> MFKNAKEFVQYANKLKTLREKKLNGVSIYVCVGTGCTAKGALKVYSAFEEELKKRNLLGQVTLEKIDDDKVTLNRTGCCGRCSSGPLVKIMPYRFFYSNVAPEDVPEIVDRTVLKGEPIERLFLTDPLTGEKVPRIEDTTLFKNQDFYIMEAIGESECDSIEDYIARSGYESLVKALTSMTPEEIIETVKASGLRGRGGGGFPTGLKWEFTRKAQGDIKFVVCNGDEGDPGAFMNRTLLERDPHLVLEGMIIAGYAVGAQKGYAYIRAEYPFAVKMFKKAIEDARKLGLLGENILGTGFSFDLEVKEGAGAFVCGEETALLASIEGKRGMPRPKPPFPAQSGLWGKPTLINNVETYANIPRILRDGVENYRKRGTENSPGTKMFSVAGPLKATGIIEVEFGTTLRDIIYNICGGFVEGEEFKAVQIGGPSGACLSEDFIDMPLDYDTLKKADAMVGSGGIVVITKKTCMVEVARFFLDFTKRESCGKCVPCREGTMQA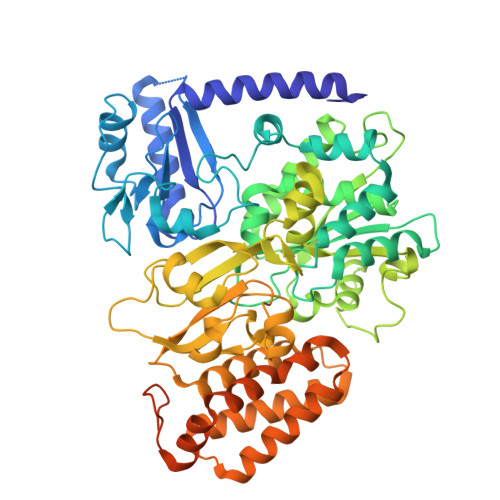YNILEKFTHGKATYEDLKTLEHLSKTIKTASLCGLGKTAPNPILSTLKLFREEYIAHIEGECPSGMCTAFKKYVINPDICKGCGLCARSCPQNAITGERGKPYTIDQEKCVKCGLCASKCPFKAIELV aaTHEP1, the gene product of aq_1292 from Aquifex aeolicus, shows sequence homology to proteins from most thermophiles, hyperthermophiles, and higher organisms such as man, mouse, and fly. In contrast, there are almost no homologous proteins in mesophilic unicellular microorganisms. aaTHEP1 is a thermophilic enzyme exhibiting both ATPase and GTPase activity in vitro. Although annotated as a nucleotide kinase, such an activity could not be confirmed for aaTHEP1 experimentally and the in vivo function of aaTHEP1 is still unknown. The crystal structure of aaTHEP1 uncovered a modified RecA-like fold.

Analysis of its nucleotide loading state using HPLC revealed that it was partially loaded with ADP (approx. 30%, data not shown). It was crystallized using PEG3350 as precipitant in the presence of KH2PO4 and crystals diffracted up to 1.4 Å using synchrotron radiation. 172 amino acid residues, 249 water molecules, one phosphate, one magnesium and two sodium ions were included in the model. No electron density was found for residues D38-K43 which are part of a disordered loop. aaTHEP1 consists of a single compact domain confirming the gel filtration experiments as well as the resistance of aaTHEP1 to limited proteolysis. All nine strands form a single sheet in topological order 918723465 wherein a five-stranded parallel and a four-stranded antiparallel region can be distinguished. In contrast, as it is the case for both aaTHEP1 and the RecA superfamily, the ASCE-proteins contain an additional strand between and a catalytic essential glutamate (E107 in aaTHEP1) within the Walker B motif, thus indicating that aaTHEP1 neither belongs to the group of GTPases nor to the kinase family. No electron density for an ADP molecule was found indicating that only the nucleotide-free protein crystallized. However, we found electron density for a phosphate ion in the putative nucleotide binding site where the β-phosphate of the nucleotide is expected. In the nucleotide free aaTHEP1, there is also a magnesium ion at the corresponding position which is octahedrally coordinated to the hydroxyl group of T14 of the P-loop, a phosphate oxygen and four water molecules. To detect putative binding sites of aaTHEP1, we colour coded the surface of aaTHEP1 with respect to the conservation of exposed amino acids. As can be seen in Figure 5, there is only one highly conserved region located in and around a cleft of the protein surface which includes the Walker A motif (P-loop).

> MKIIITGEPGVGKTTLVKKIVERLGKRAIGFWTEEVRDPETKKRTGFRIITTEGKKKIFSSKFFTSKKLVGSYGVNVQYFEELAIPILERAYREAKKDRRKVIIIDEIGKMELFSKKFRDLVRQIMHDPNVNVVATIPIRDVHPLVKEIRRLPGAVLIELTPENRDVILEDILSLLER> KQFVTVFYGIPAWRNASIPLFCATKNRDTWGTIQCLPDNDDYQEIALNVTEAFDAWNNTVTEQAVEDVWNLFETSIKPCVKLTPLCVAMNCTRNMTTSTGTTDTQNITIINDTSPCVRADNCTGLKEEEMVDCQFNMTGLERDKRKQYTEAWYSKDVICDNNTSSRSKCYMNHCNTSVITESCDKHYWDAMRFRYCAPPGFALLRCNDTNYSGFAPNCSKVVAATCTRMMETQSSTWFGFNGTRAENRTYIYWHGKNNRTIISLNNFYNLTMHCKRPGNKTVLPIMSGFKFHSKPVINKKPRQAWCWFKGEWKEAMQEVKETLAKHPRYKGNRSRTENIKFKAPGRGSDPEAAY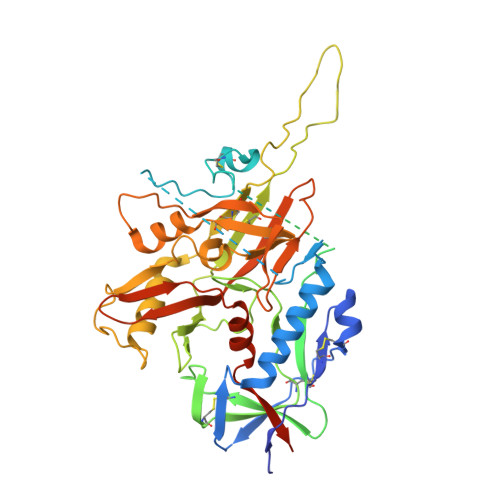MWTNCRGEFLYCNMTWFLNWVDNRTGQKQRNYAPCHIRQIINTWHRVGKNVYLPPREGELTCNSTVTSIIANIDTGDQTDITFSAEVAELYRLELGDYKLVEITPIGFAPTSVKRYSSAHQRHTR allyl-cysteine | C6 H11 N O2 S | 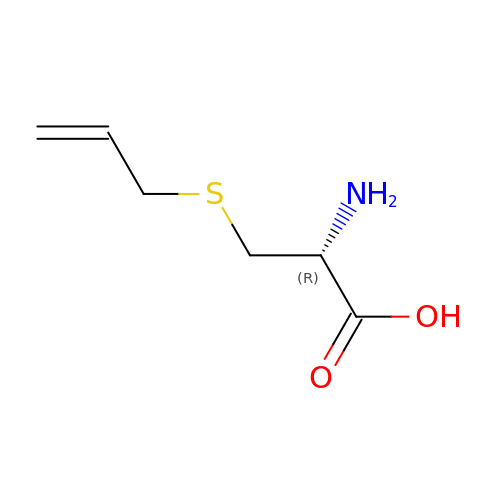ZFAHNWWNDFHPOH-YFKPBYRVSA-N>[2x]MVPISPIETVPVKLKPGMDGPKVKQWPLTEEKIKALVEICTEMEKEGKISKIGPENPYNTPVFAIKKKDSTKWRKLVDFRELNKRTQDFWEVQLGIPHPAGLKKKKSVTVLDVGDAYFSVPLDEDFRKYTAFTIPSINNETPGIRYQYNVLPQGWKGSPAIFQSSMTKILEPFKKQNPDIVIYQYMDDLYVGSDLEIGQHRTKIEELRQHLLRWGLTTPDKKHQKEPPFLWMGYELHPDKWTVQPIVLPEKDSWTVNDIQKLVGKLNWASQIYPGIKVRQLSKLLRGTKALTEVIPLTEEAEL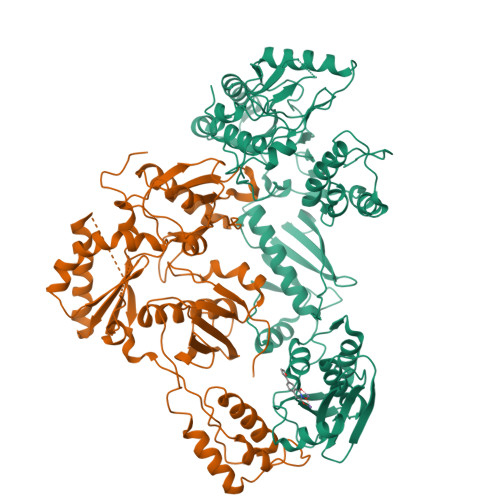ELAENREILKEPVHGVYYDPSKDLIAEIQKQGQGQWTYQIYQEPFKNLKTGKYARMRGAHTNDVKQLTEAVQKITTESIVIWGKTPKFKLPIQKETWETWWTEYWQATWIPEWEFVNTPPLVKLWYQLEKEPIVGAETFYVDGAANRETKLGKAGYVTNKGRQKVVPLTNTTNQKTELQAIYLALQDSGLEVNIVTDSQYALGIIQAQPDKSESELVNQIIEQLIKKEKVYLAWVPAHKGIGGNEQVDKLVSAG;>GPISPIETVPVKLKPGMDGPKVKQWPLTEEKIKALVEICTEMEKEGKISKIGPENPYNTPVFAIKKKDSTKWRKLVDFRELNKRTQDFWEVQLGIPHPAGLKKKKSVTVLDVGDAYFSVPLDEDFRKYTAFTIPSINNETPGIRYQYNVLPQGWKGSPAIFQSSMTKILEPFKKQNPDIVIYQYMDDLYVGSDLEIGQHRTKIEELRQHLLRWGLTTPDKKHQKEPPFLWMGYELHPDKWTVQPIVLPEKDSWTVNDIQKLVGKLNWASQIYPGIKVRQLSKLLRGTKALTEVIPLTEEAELELAENREILKEPVHGVYYDPSKDLIAEIQKQGQGQWTYQIYQEPFKNLKTGKYARMRGAHTNDVKQLTEAVQKITTESIVIWGKTPKFKLPIQKETWETWWTEYWQATWIPEWEFVNTPPLVKLWYQ[2x]>[10x]MNIIQGNLVGTGLKIGIVVGRFNDFITSKLLSGAEDALLRHGVDTNDIDVAWVPGAFEIPFAAKKMAETKKYDAIITLGTVIRGATTHYD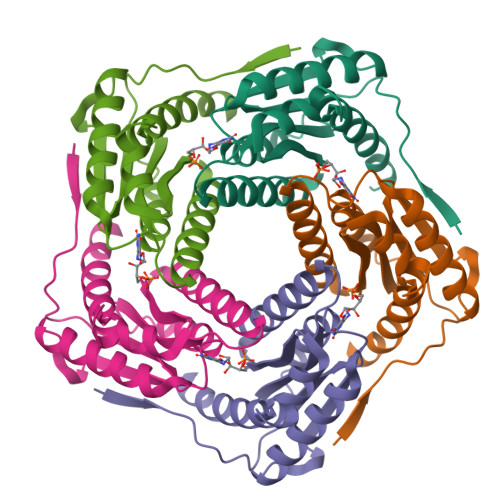YVCNEAAKGIAQAANTTGVPVIFGIVTTENIEQAIERAGTKAGNKGVDCAVSAIEMANLNRSFE>MAHHHHHHMSETKNSEYFIELEEKHGAHNYHPLPVVLDRGEGVFVWDVEGKKYYDFLSAYSAVNQGHSHPKIVEALVEQASKLALTSRAFYNSKLGEYEQKITSLLGFDKVLPMNSGAEAVETAVKLARKWSYEVKGIAENAAKIIVCENNFHGRTTTIVSFSNDPDANQNYGPFTPGFIRIPYNDIAALEEVLSKEAGNIAAFLVEPIQGEAGVYVPNEGFLKQSSELCKKHNVLFIADEVQTGIARTGKLIACHHEDVQPDILILGKALSGGMYPVSAVLANNNIMDVIKPGQHGSTFGGNPLACAVAMAALDVVQDEKLSERAEKLGNLFRSEIEKLIEKTDLITKVRGKGLLNAILINDTPDSS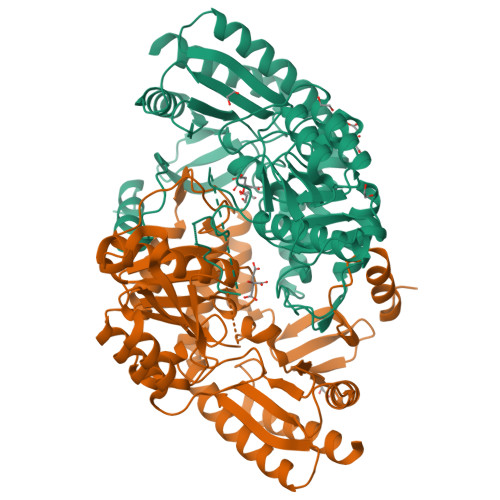TAWNLCLALKENGLLAKPTHGNIIRLAPPLVITEEQLLDCVKIIEKTILEF[2x]>DNQFYSVEVGDSTFTVLKRYQNLKPIGSGAQGIVCAAYDAVLDRNVAIKKLSRPFQNQTHAKRAYRELVLMKCVNHKNIISLLNVFTPQKTLEEFQDVYLVMELMDANLCQVIQMELDHERMSYLLYQMLCGIKHLHSAGIIHRDLKPSNIVVKSDCTLKILDFGLARTAGTSFMMTPYVVTRYYRAPEVILGMGYKENVDIWSVGCIMGEMVRHKILFPGRDYIDQWNKVIEQLGTPCPEFMKKLQPTVRNYVENRPKYAGLTFPKLFPDSLFPADSEHNKL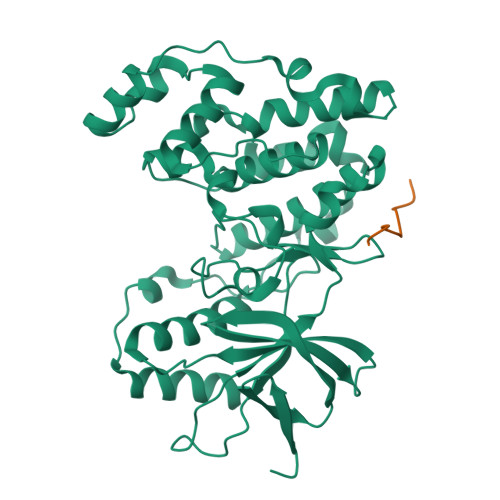KASQARDLLSKMLVIDPAKRISVDDALQHPYINVWYDPAEVEAPPPQIYDKQLDEREHTIEEWKELIYKEVMN[2x];>[2x]VVRPGSLDLP> SRSESSIESFFARGACVTIMTVDNPASTTNKDKLFAVWKITYKDTVQLRRKLEFFTYSRFDMELTFVVTANFTETNN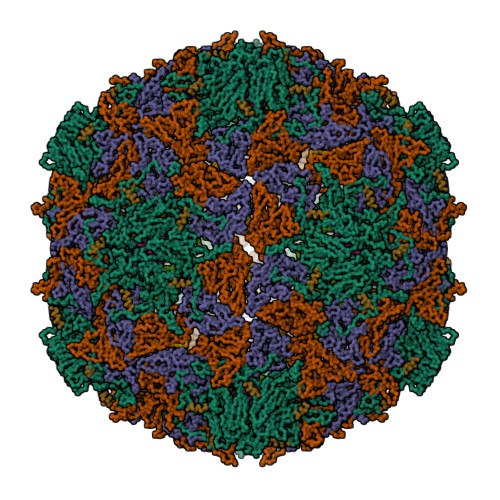GHALNQVYQIMYVPPGAPVPEKWDDYTWQTSSNPSIFYTYGTAPARISVPYVGISNAYSHFYDGFSKVPLKDQSAALGDSLYGAASLNDFGILAVRVVNDHNPTKVTSKIRVYLKPKHIRVWCPRPPRAVAYYGPGVDYKDGTLTPLSTKDLTTY;> AANSVVAYGRWPEYLRDSEANPVDQPTEPDVAACRFYTLDTVSWTKESRGWWWKLPDALRDMGLFGQNMYYHYLGRSGYTVHVQCNASKFHQGALGVFAVPEMCLAGDSNTTTMHTSYQNANPGEKGGTFTGTFTPDNNQTSPARRFCPVDYLLGNGTLLGNAFVFPHQIINLRTNNCATLVLPYVNSLSIDSMVKHNNWGIAILPLAPLNFASESSPEIPITLTIAPMCCEFNGLR;> DTMIPFDLSATKKNTMEMYRVRLSDKPHTDDPILCLSLSPASDPRLSHTMLGEILNYYTHWAGSLKFTFLFCGSMMATGKLLVSYAPPGADPPKKRKEAMLGTHVIWDIGLQSSCTMVVPWISNTTYRQTIDDSFTEGGYISVFYQTRIVVPLSTPREMDILGFVSACNDFSVRLLRDTTHI;> GLPVMNTPGSNQ;> LTADNFQSPCALPEFDVTPPIDIPGEVKNMMELAEI;> VLQLTLGNSTITTQ;> PALTAVETGAT> MAISKTNGQSKPKRKTEVPGQALGYSLQFTLLTHLLLQAPEGSLCSLEVLDDVAQENNSGDIKFIQSASALTANPAADRAKSLWKTLSNWIDLATSPDFEVEKAIFELYVSRPVEGSIVKKFNEAKTPEDAQEAITHARTELWGDSPHFTLKDGISKEISKYVEKVFTADQNLLQRLICNFQLTLGSGSPQADLEACVRSHPVSPSKVSDITNYLCGKVKRHIDMLLEAEKPAVIARDDFYTWYKAYVQKIDRQMVLSSRAQAPVKEKAQEYLPDKFVQQLEIIGLPYEEILGAISDYLMASFDRTDWAARGEVDETSFDDLDTALQRTWKNKQRICGLTHSEKSEQDQGKLLYFECMQFNIPLQAMSPPSHFIPGCYHILADSLAVGWHPNYTT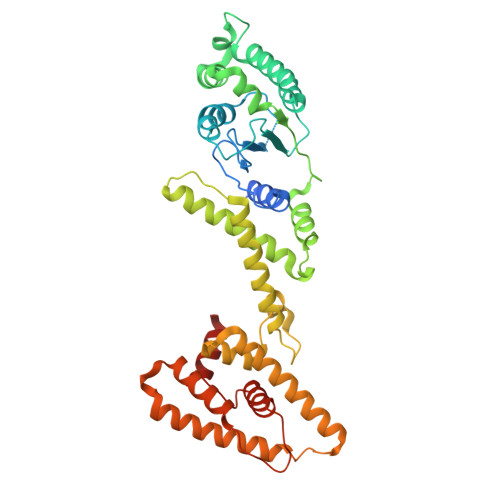QLKNKKVA>[2x]MRGSHHHHHHGSNVAKNNLKNNKDIERKEKIIILGSGWGGFNFLLNIDFKKYDVTLISPRNYFTFTPLLPCLCSGTLSVNVCTESIRNFLRKKNGYCGNYLQLECTDVFYEDKYINCIDIENNKVKLFYDYLIIAVGAKTNTFNINGVDKYAYFVKDIDDALKIRKKFLDILEKCTLPNISNEEKKKMLHVAVVGGGPTGVEVTAEFADFINKEVKINYKDIFNFISISIIEGGNNLLPTFTQNISDFTKENFHNLNINVLTNYYVIDVDKHSFHIQSSLNK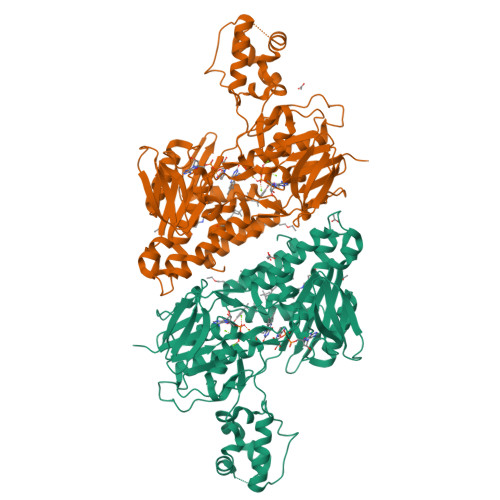NEKKKLSYGLLIWASGLAQTTLIQKFLKTIPVQANNAILKVDEKLRVIGIPSNNIYAIGDCKKIQPKLLHEHTNEIIKILTGNKLTSEALKLKQSELTKTFPQLSISKWDYEKNKKGEMTPQQFHDYLFEIDKNYKSPTPTAQNAKQEAYYLSNVFNNFIHTNQKFNIPSFIEKWKGSLAYIGNHQVVADLPYYELKGGRFSSTFWKVVYIQLLLSWKSRFHFFIDFIKTKWYGRPFIK NleE, a virulence effector from EPEC, is a SAM-dependent methyltransferase that modifies a zinc-finger cysteine in TAB2/3 in the NF-κB pathway. We recently discovered that NleE is a SAM-dependent methyltransferase that modifies a cysteine in the NZF domains of TAB2/3, thereby disrupting ubiquitin-chain sensing of TAB2/3 and abolishing NF-κB-mediated proinflammatory responses. NleE-catalyzed cysteine methylation of TAB2/3 is the first example of enzyme-catalyzed protein cysteine methylation, representing a novel mechanism in regulating signal transduction in eukaryotes. NleE harbors no sequence homology to known methyltransferases.

Wild-type NleE yielded poor crystals, but NleE K181A protein, out of 15 Lys-to-Ala mutants designed to improve the crystallization, produced sufficient-quality crystals in the C2 space group. A model obtained from 2.6-Å diffraction data collected on the selenomethionine (Se-Met) protein was further refined and a final resolution of 2.3 Å was achieved. Despite the presence of four NleE in an asymmetric unit (chain A–D), NleE was exclusively a monomer in solution as judged by gel filtration chromatography analysis. The structure of NleE (residues 21–220: residues 1–20 and 220–224 lacked electron density) adopts α/β doubly wound topology with a central three-stranded anti-paralleled β-sheet (β1–β3) sandwiched by α-helices (α1–α10). β1–β3 are arranged in the left-right-middle order, which, together with the flanking α-helices (α8–α10), generates a deep and narrow cavity on the left side of NleE. The SAM molecule fits snugly into the cavity, which buries 2374 Å2 solvent accessible surface area, corresponding to 76% of the total surface area of SAM and leaving the rest of 24% exposing to the solvent. The interior of the SAM-binding cavity is filled with hydrophobic side chains, but polar interactions appear to play a key role in riveting the SAM into the cavity. Specifically, the α-carboxylic group of the amino acid moiety of the SAM is coordinated by the side chain of Arg107 situated on a loop connecting β1 and α6. The hydroxyl group of the ribose of the SAM is hydrogen-bonded with the side-chain carboxylic group of Glu191. The adenine ring of SAM is oriented by the aromatic ring of Tyr212 residing at α10 (residues 206–219) through a π-π stacking interaction. Remarkably, the overall architecture of NleE does not resemble any of the five families, thus representing a completely novel class of methyltransferases.

>[4x]MINPVTNTQGVSPINTKYAEHVVKNIYPEIKHDYFNESPNIYDKKYISGITRGVAELKQEEFVNEKARRFSYMKTMYSVCPEAFEPISRNEASTPEGSWLTVISGKRPMGQFSVDSLYNPDLHALCELPDICCKIFPKENNDFLYIVVVYRNDSPLGEQRANRFIELYNIKRDIMQELNYALPELKAVKSEMIIAREMGEIFSYMPGEIDSYMKYINNKLSKIE>SAKEKFTSLSPAEFFKRNPELAGFPNPARALYQTVRELIENSLDATDVHGILPNIKITIDLIDDARQIYKVNVVDNGIGIPPQEVPNAFGRVLYSSKYVNRQTRGMYGLGVKAAVLYSQMHQDKPIEIETSPVNSKRIYTFKLKIDINKNEPIIVERGSVENTRGFHGTSVAISIPGDWPKAKSRIYEYIKRTYIITPYAEFIFKDPEGNVTYYPRLTNKIPKPPQEVKPHPYGVDREEIKILINNLKRDYTIKEFLVNEFQSIGDTTADKILELAGLKPNKKVKNLTEEEITRLVETFKKYEDFRSPSADSLSVIGEDLIELGLKKIFNPDFAASITRKPKAYQGHPFIVEAGVAFGGSIPVGEEPIVLRYANKIPLIYDEKSDVIWKVVEELDWKRYGIE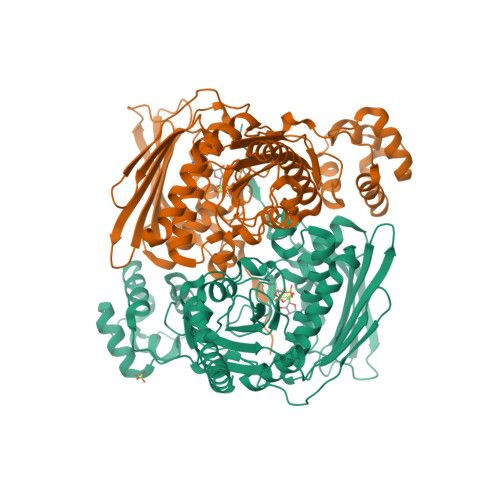SDQYQMVVMVHLCSTKIPYKSAGKESIAEVEDIEKEIKNALMEVARKLKQYLSEKRKEQEAKKKLLA[2x]> MEKKTIVLGVIGSDCHAVGNKILDHAFTNAGFNVVNIGVLSPQENFIKAAIETKADAILVSSLYGQGEIDCKGL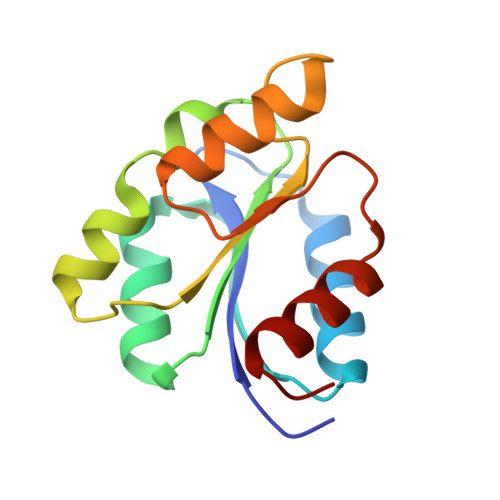RQKCDEAGLEGILLYVGGNIVVGKQHWPDVEKRFKDMGYDRVYAPGTPPEVGIADLKKDLNIE>MKEQLEDVLDTLTDREENVLRLRFGLDDGRTRTLEEVGKVFGVTRERIRQIEAKALRKLRHP[2x];>MKLKILDKDNATLNVFHRN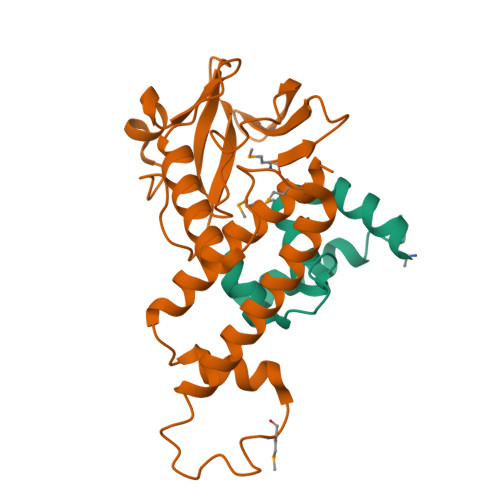KEHKTIDNVPTANLVDWYPLSNAYEYKLSRNGEYLELKRLRSTLPSSYGLDDNNQDIIRDNNHRCKIGYWYNPAVRKDNLKIIEKAKQYGLPIITEEYDANTVEQGFRDIGVIFQSLKTIVVTRYLEGKTEEELRIFNMKSEESQLNEALKESDFSVDLTYSDLGQIYNMLLLMKKISK[2x]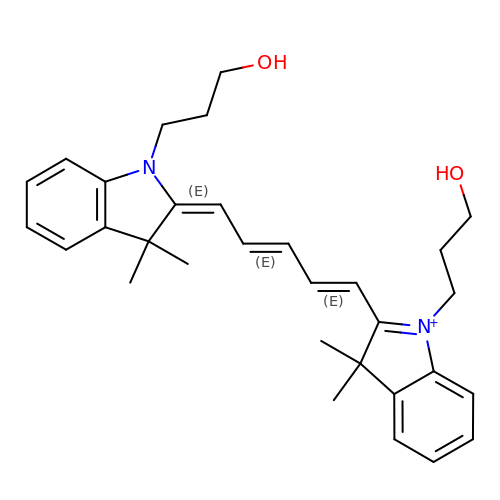1-(3-hydroxypropyl)-2-{(1E,3E,5E)-5-[1-(3-hydroxypropyl)-3,3-dimethyl-1,3-dihydro-2H-indol-2-ylidene]penta-1,3-dien-1-yl}-3,3-dimethyl-3H-indolium | C31 H39 N2 O2 | VFBDPICHYNKCQJ-UHFFFAOYSA-N>MEPGPTAAQRRCSLPPWLPLGLLLWSGLALGALPFGSSPHRVFHDLLSEQQLLEVEDLSLSLLQGGGLGPLSLPPDLPDLDPECRELLLDFANSSAELTGCLVRSARPVRLCQTCYPLFQQVVSKMDNISRAAGNTSESQSCARSLLMADRMQIVVILSEFFNTTWQEANCANCLTNNSEELSNSTVYFLNLFNHTLTCFEHNLQGNAHSLLQTKNYSEVCKNCREAYKTLSSLYSEMQKMNELENKAEPGTHLCIDVEDAMNITRKLWSRTFNCSVPCSDTVPVIAVSVFILFLPVVFYLSSFLHSEQKKRKLILPKRLKSSTSFANIQENSNLEHHHHHHHH[2x];>MASDYKDDDDKASDEVDAGTMANVSKKVSWSGRDRDDEEAAPLLRRTARPGGGTPLLNGAGPGAARQSPRSALFRVGHMSSVELDDELLDPDMDPPHPFPKEIPHNEKLLSLKYESLDYDNSENQLFLEEERRINHTAFRTVEIKRWVICALIGILTGLVACFIDIVVENLAGLKYRVIKGNIDKFTEKGGLSFSLLLWATLNAAFVLVGSVIVAFIEPVAAGSGIPQIKCFLNGVKIPHVVRLKTLVIKVSGVILSVVGGLAVGKEGPMIHSGSVIAAGISQGRSTSLKRDFKIFEYFRRDTEKRDFVSAGAAAGVSAAFGAPVGGVLFSLEEGASFWNQFLTWRIFFASMISTFTLNFVLSIYHGNMWDLSSPGLINFGRFDSEKMAYTIHEIPVFIAMGVVGGVLGAVFNALNYWLTMFRIRYIHRPCLQVIEAVLV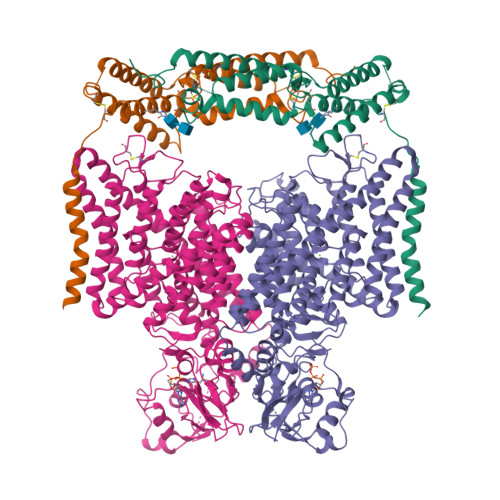AAVTATVAFVLIYSSRDCQPLQGGSMSYPLQLFCADGEYNSMAAAFFNTPEKSVVSLFHDPPGSYNPLTLGLFTLVYFFLACWTYGLTVSAGVFIPSLLIGAAWGRLFGISLSYLTGAAIWADPGKYALMGAAAQLGGIVRMTLSLTVIMMEATSNVTYGFPIMLVLMTAKIVGDVFIEGLYDMHIQLQSVPFLHWEAPVTSHSLTAREVMSTPVTCLRRREKVGVIVDVLSDTASNHNGFPVVEHADDTQPARLQGLILRSQLIVLLKHKVFVERSNLGLVQRRLRLKDFRDAYPRFPPIQSIHVSQDERECTMDLSEFMNPSPYTVPQEASLPRVFKLFRALGLRHLVVVDNRNQVVGLVTRKDLARYRLGKRGLEELSLAQT[2x]5-[[3-(aminomethyl)phenyl]methyl]-3-pentyl-quinolin-2-amine | 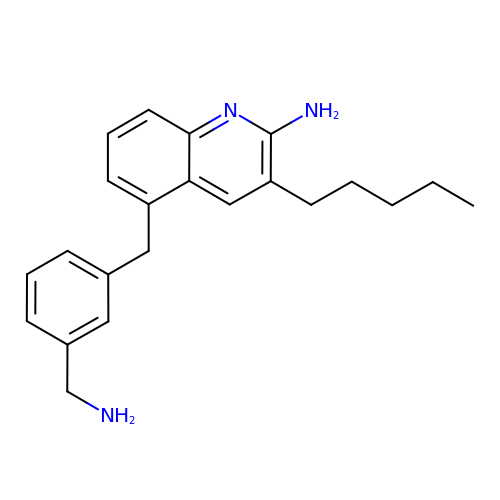C22 H27 N3 | MJTYFAQITQYOAV-UHFFFAOYSA-N> MGTKERILEVSKELFFEKGYQGTSVEEIVKRANLSKGAFYFHFKSKEELITEII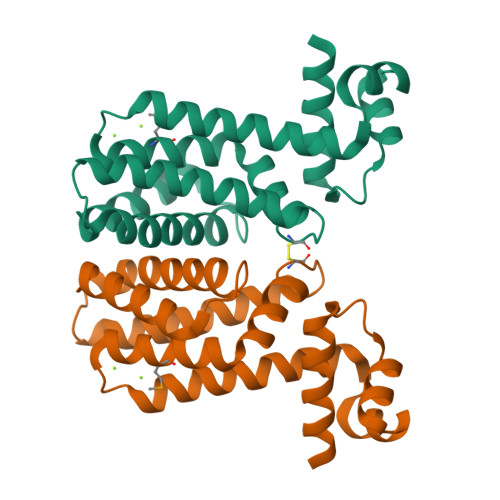ERTHKKIISLFEENKEKTPEELLEMFLEVLYREKKVVYIFLFDLLCSEKFRNIYFEKIEDAKRRFEKFLEKHFPSKAEILSEIILGFLRQLILHYVIKEERELPFLKEKLREGLKLIFEGVKKCG>MKDNSTSAVSSWLGYKIQ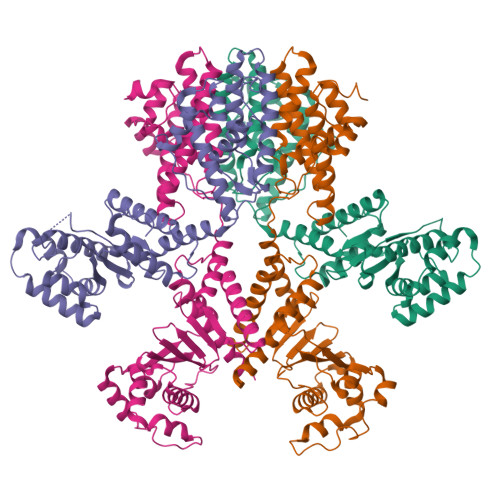EYRLTQRLLEANNSSCIGFEILDDLEEHTGSTSTFEQDKISTTGRNIVSNHSKDLWKTLSNWMDLIDSGEIDVDNTIFLLFTNKRCHSEVLQLLSTSQATEEASKAFDEILKIVSHPSPSIANYLNNFSKSKTDACRLISKFTYIYGSGSAPHDLRESYKLHRLGALEEHLDEIMYEILGWVSDVLTLAAEKRQPTIVRAKDFGARLGEIESKYRQKTILNYFCNRSSESEDVQNTIKDAPNYIKQLNLINVDDSELEEAAIANLETKDAVVEWTLNGDVQDYSYRYYQRELRRCWGIQKQKIHLDFNGRPETEVGQRLYIECLNNVTRYYLENKKVGDFFAHGTLHSMADKLTIGWHPEFDKKLGDPDA[4x]>[3x]EAEFQSQSLCAQYASYTGSTYGLNNNLWGEASGSGSQCTYLNSASSSSINWYTTWTWSGNANEVKSYA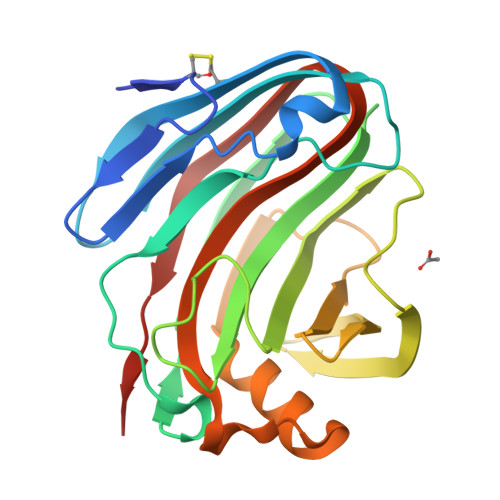NSQLLSFTKKYVSNIGSIPTTAQWSLSNTGVNADVAYDLFTSSNINHVTYSGDYELMIWLGRYGSIQPIGSQIATATIAGYTWEVWYGGSSSQWTYSYVASSPITSFSGDIIDFFHDMTNNHGFPASSQYLIDLQFGTEPFTGGPTTLTVSSWSASVNLDHHHHHH> SNAFEEVRDFFYDRNNYI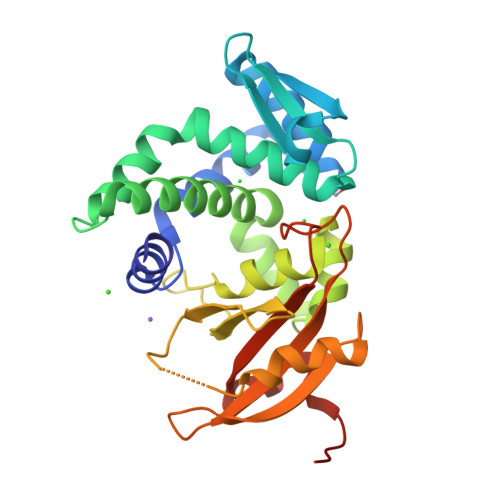HDLDMAAERMFTESGMRTGGLDIQLAELMRDRFGISVVIDDNLPDTAKRRYHPDTKVLRVAHWLMPGQRAFQIATQLALVGQSDLISSIVATDDQLSTEARGVARIGLANYFAGAFLLPYREFHRAAEQLRYDIDLLGRRFGVGFETVCHRLSTLQRPRQRGIPFIFVRTDKAGNISKRQSATAFHFSRVGGSCPLWVVHDAFAQPERIVRQVAQMPDGRSYFWVAKTTAADGLGYLGPHKNFAVGLGCDLAHAHKLVYSTGVVLDDPSTE> GGSEVRILLLGLDNAGKTTLLKQLASEDISHITPTQGFNIKSVQSQGFKLNVWDIGGQRKIRP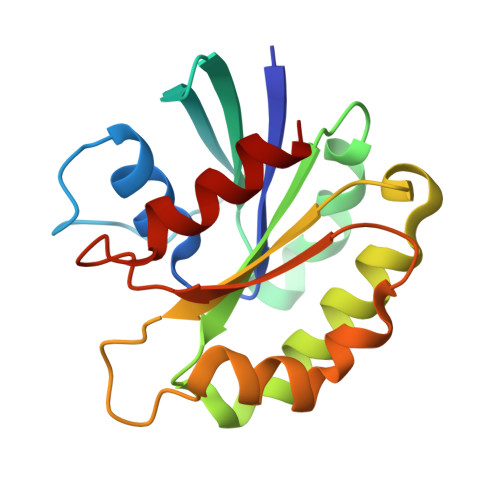YWRSYFENTDILIYVIDSADRKRFEETGQELTELLEEEKLSCVPVLIFANKQDLLTAAPASEIAEGLNLHTIRDRVWQIQSCSALTGEGVQDGMNWVCKNV>HHHHHHSSGLVPRGSHMQTTTVYSLEDLLPYLKQDNVDVKLAPGTYNVNGFDVGEDRLFSTTPLFLFEGSNSTYDFTDVKLNINTVVLTKFGNNEVNEIQILGNNNVLKNLKLEDIGTTAPSNRAQSIVIDGRDNRIEGFHLTIRGSYPYGYGDAFGKGGGSVINHRKHSGVLIRGLRNHLKDCTIISRSYGHIVFMQAASYPTVEGCYIEGEMRSTDDMLAEEGTGSPADKVDFMTVWGYKLPAGYMMSLQEGGIAAYNAGTTYIDGVEIQRATDNPTVLNCTIKNARTGVTLAHANGTKYVEGCTVLGCENGYSIGSGTVVNCGADAIYGPVFKNTYGSDKGYNADITILPPSDAYYNGHDAVAYIGGSNHNLTFRSEITEIPSNLKIMVSGDLQGLRVLHGSNPSQNNFAGTNIVLRNLTNFPVDLHSDSSNITVTSCDTDNITDNGTNNSIEAIDCDSD[2x]

FdlA from Flavobacterium sp. SA-0082 is an endo-type fucoidan-degrading enzyme that cleaves the sulfated fuco-glucuronomannan (SFGM) through a lytic mechanism. We show that the FdlA-NTD adopts a right-handed parallel β-helix fold, and possesses a substrate binding site composed of a long groove and a unique alkaline pocket. Our structural, biochemical, and enzymological analyses strongly suggest that FdlA-NTD utilizes catalytic residues different from other β-helix polysaccharide lyases, potentially representing a novel polysaccharide lyase family. Here, we report crystal structures and enzymological characterization of wild type (WT) and eight single mutants of the catalytic N-terminal domain (NTD) of FdlA, revealing its unique substrate binding pocket and identifying the key catalytic residues.

We first measured the enzymatic activity of 12 mutants and found that eight of them (D137A, K141A, H176A, F179A, E236A, R240A, Y242A, and Y242F) almost completely abolished their activities, H279A mutant retained approximately 65% of the activity compared with WT, while mutations of Asn243, Arg272, and Tyr322 to Ala only negligibly affect their activities. Two positively charged residues Lys141 and Arg240 have their side chains pointing closely to the C-5 atom at the +1 subsite, hence are potential candidates for a catalytic base. In contrast, the R240A mutant exhibits visible structural changes around the active site. Specifically, the Try242 residue was rotated approx. 90 degrees, and shifted toward Ala240. As it constitutes the catalytic acid, the hydroxyl group of the Tyr242 side chain is essential for the enzymatic activity, and its improper positioning may severely affect the catalysis of the enzyme. These structures suggested that the loss of activity of the R240A mutant may be due to the shift of the Tyr242 side chain. Based on our structural and docking models, several positively charged residues such as Arg240, His176, and Lys141, located near the +1 subsite, potentially serve as neutralizers in FdlA-NTD, weakening the negative charge of the C-5 carboxyl group at +1 subsite, and making the C-5 proton susceptible to the attack by a Brønsted base. Next, the positively charged residues including Arg240 and His176, which are located near the +1 subsite, neutralize the C-5 carboxyl group of D-GlcUA at +1 subsite, thus reducing the pKa of the C-5 proton, making it more susceptible to the attack by a base.> QFAKPEDAVKYRQSAGTLMASHFGRMTPVVKGQAPYDAAQIKANVEVLKTLSALPWAAFG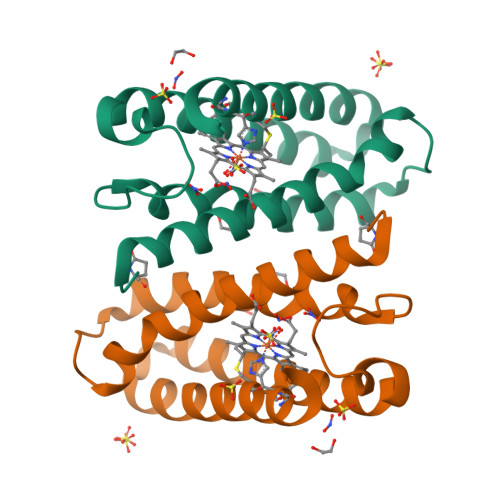PGTEGGDARPEIWSDAASFKQKQQAFQDNIVKLSAAADAGDLDKLRAAFGDVGASCKACHDAYRKKK(1R,3R,7E,9beta,17beta)-9-butyl-17-[(2R)-6-hydroxy-6-methylheptan-2-yl]-9,10-secoestra-5,7-diene-1,3-diol 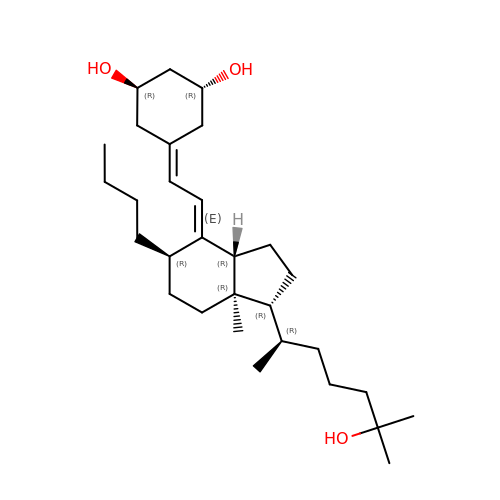| C30 H52 O3 | HGPWGYLACPHOSW-ZOBUFXTASA-N>GKAGVLKLPIESIHRDKDQPRTYFDEEKLKELSESIKAQGVLQPILVRKDGDGYRIIAGERRWRASQAAGLKEVPAIVRDVTEVQAFELALVENLQRADLNPIEEAEGYKRLVDEFKLTQEQVSVRVGKERSTVANALRLLALPTDVKGMVADGSLSMGHARALLGVPRLPELQNLAKQVADKK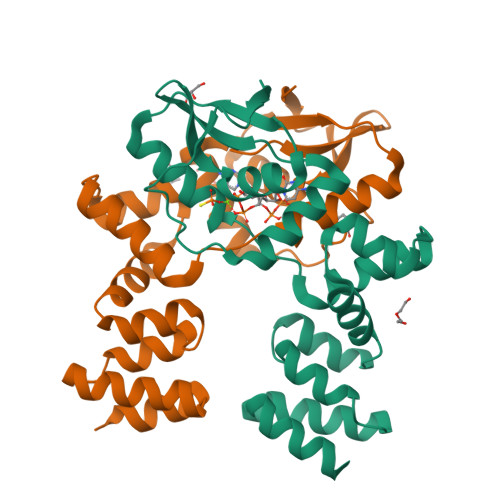LSVRDTERLVQQSRSSGKKDAGKAAPKQS[2x]> II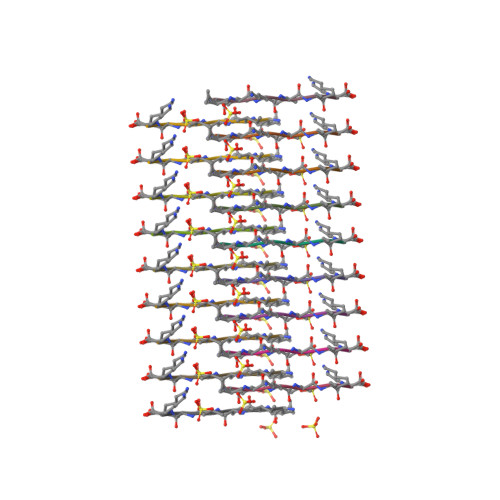KVIK> DSFINIFVSIDKDGTNVISYPELEQYVAENNLDPSMVEKWKQLFDPDNTGSITLETFCSKLGLKPAEIIDFREQKGLHAA

Tegumental protein of 20.8 kDa from Clonorchis sinensis elicits IgA immune responses in the host and does not cause an IgG response. For this reason, we named the 20.8-kDa tegumental protein from Clonorchis sinensis as CsTAL3. The interesting thing is that similar results were reported for SmTAL2 and FhCaBP2, 40. Both proteins belong to the TAL protein family of the class of fluke proteins that consist of a calmodulin like domain (or N-terminal domain) and a DLC-like domain (or C-terminal domain) as in CsTAL3. In this work, we determined 2.6 Å crystal structure of the DLC-like domain (amino acid [aa] positions 83–177) and 1.3 Å crystal structure of the calmodulin like domain (aa positions 1–81) of CsTAL3.

Due to cleavage of the full-length protein, we had grown a crystal of the calmodulin like domain (aa 1–81) of CsTAL3. The initial phase determination and model building were carried out by the SAD method with an anomalous signal of one selenomethionine. The structure of the calmodulin like domain is composed of five α-helices. The α1 to α4 helices are classical EF-hand motifs where two helix-loop-helix structures and two short antiparallel β-sheets (β1 and β2) are connecting the Ca2+-binding loops. Ca2+-binding motif 1 (CB1, residues 12–23) is a Ca2+-binding loop that contains 12 partially conserved residues starting with N-terminal aspartate and ending with C-terminal glutamate as in the EF-hand motif of other calmodulin like proteins. One Ca2+ ion binds to CB1 via D12, D14, T16, V18, E23, and a water molecule (positions X, Y, Z, −Y, −Z, and −X, respectively) in a geometrical pattern of a pentagonal bipyramid. Other residues bind a Ca2+ ion via their side chain carboxyl groups, but V18 (–Y position) binds to a Ca2+ ion via its main-chain carbonyl oxygen atom. Moreover, CB2 structure appears to be similar to that of CB1, but a Ca2+ ion is absent in our structure. A significant difference is that the –Z position of CB1. This position is glutamate in the other EF-hand motif, but the –Z position of CB2 is threonine (T57). The molecule shows structural similarities with the calmodulin like domain of a family of soluble Ca2+ sensor Kv-channel-interacting proteins (KChIPs) and of the short Ca2+-binding mitochondrial carrier (SCaMC) with r.m.s. deviation 1.8 Å and 2.8 Å, when 60 Cα and 62 Cα atoms are aligned, and DALI server Z-scores 8.2 and 8.146, respectively.Amblyomin-X is a Kunitz-type FXa inhibitor identified through the transcriptome analysis of the salivary gland from Amblyomma sculptum tick. This protein consists of two domains of equivalent size, triggers apoptosis in different tumor cell lines, and promotes regression of tumor growth, and reduction of metastasis. Amblyomin-X is a Kunitz-like FXa inhibitory protein of 106 amino acids and 7 cysteine residues. As a recombinant protein, Amblyomin-X inhibits Factor Xa (FXa) activity in vitro and presents the anticoagulant property in animal models.

The synthesis of two truncated (synthetic) regions of Amblyomin-X, one called the Kunitz domain which corresponds to fragments (1–57) of Amblyomin-X contains the first 6 cysteine residues, the other the C-ter domain which corresponds to fragment 58-106 in which cysteine 67 has been mutated to the Serine residue, as well as the associated peptides, were performed by solid-phase peptide synthesis (SPPS). The crystal structure of the Kunitz domain of Amblyomin-X belongs to the orthorhombic space group P212121 with two molecules in the asymmetric unit. The diffraction limit of 1.60 Å was recorded for the best data set collected. The X-ray analysis confirms that the first portion of Amblyomin-X (amino acids 1–58) possesses a typical Kunitz structure, with two α-helices and two β-sheets kept together with three disulfide bridges (Cys7-Cys58, Cys33-Cys54, Cys18-Cys41). The main difference is remarkable around the TFPI-K2 binding loop (Pro11-Thr19) where the loop of Kunitz domain of Amblyomin-X (Ala13-Glu23) is longer than those of the human TFPI-k2. The diversity between the two loops of these Kunitz domains could suggest a different interaction of Kunitz domain of Amblyomin-X with the FXa. This consideration is in agreement with the evidence that Kunitz domain of Amblyomin-X showed lower inhibitory activity against FXa than TFPI-K2. In contrast, the N-ter Kunitz domain of Amblyomin-X is not capable of crossing through the cell membrane but is associated with tumor cell cytotoxicity when it is microinjected into the cells or fused to TAT cell-penetrating peptide. No microinjection cells were used as control. This result indicates that the Kunitz domain could be responsible for cytotoxicity and its internalization is crucial for this effect.

>ANSKAVCNLPKLAGDETCSNKTEIRWYYNGTACEAFIFKGCGGNDNNFDRVDDCQRLC[2x]>[2x]M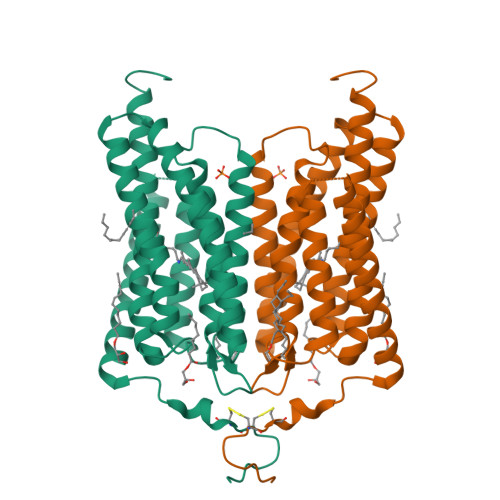DYGGALSAVGRELLFVTNPVVVQGSVLVPEDQCYCAGWIESRGTNGAQTASNVLQWLAAGFSILLLMFYAYQTWKSTCGWEEIYVCAIEMVKVILEFFFEFKNPSMLYLATGHRVQWLRYAEWLLTTPVILIHLSNLTGLSNDYSRRTMGLLVSDIGTIVWGATSAMATGYVKVIFFCLGLCYGANTFFHAAKAYIEGYHTVPKGRCRQVVTGMAWLFFVSWGMFPILFILGPEGFGVLSVYGSTVGHTIIDLMSKNCWGLLGHYLRVLIHEHILIHGDIRKTTKLNIGGTEIEVETLVEDEAEAGAVNKGTGK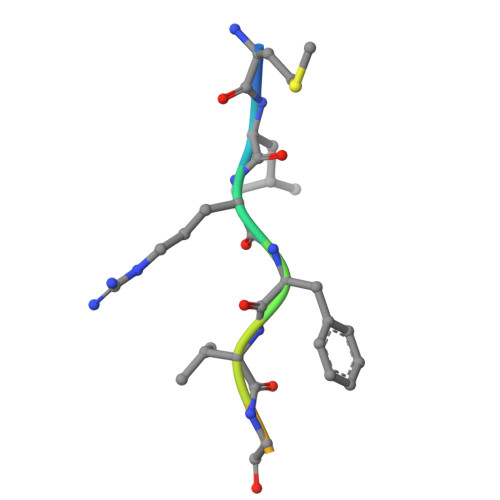> MLRFVGSRRR> QTAR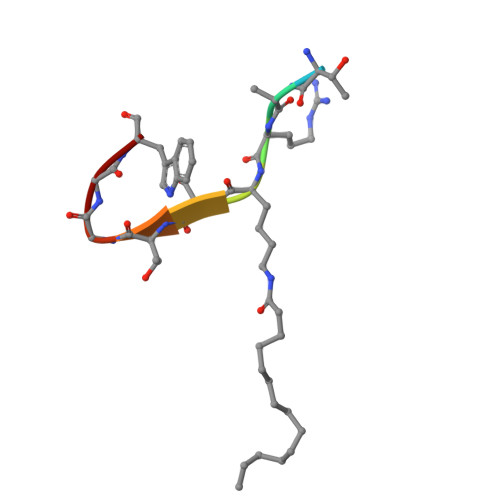XSTGGW>SNAMTATNPDYFELRHTVGFEETNLVGNVYYVNYLRWQGRCRELFLKERAPSVLAEVQEDLKLFTLKVDCEFFAEITAFDELSIRMRLSELRQTQLEFTFDY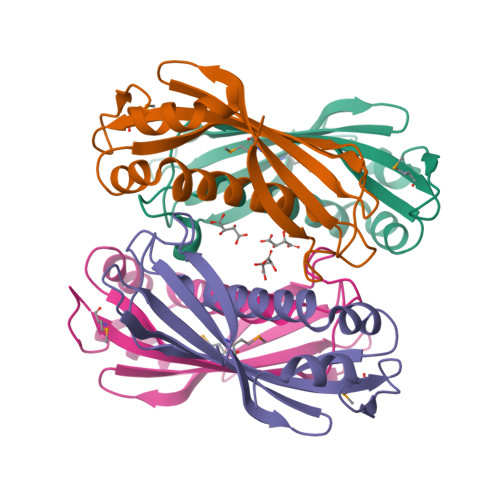IKLGDDGGETLVARGRQRIACMRGPNTATVPTLIPEALAEALAPYSDRAGSYAGRAA[8x]>GSHMNILVTGGAGFIGSHVVDKLIENGYGVIVVDNLSSGKVENLNRNALFYEQSIEDEEMMERIFSLHRPEYVFHLAAQASVAISVREPARDAKTNIIGSLVLLEKSIKYGVKKFIFSSTGGAIYGENVKVFPTPETEIPHPISPYGIAKYSTEMYLEFFAREYGLKYTVLRYANVYGPRQDPYGEAGVVAIFTERMLRGEEVHIFGDGEYVRDYVYVDDV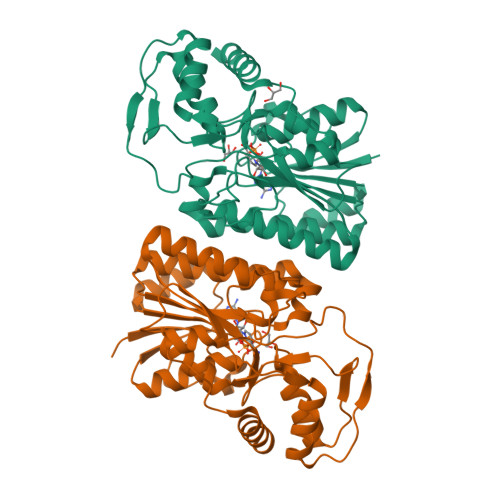VRANLLAMEKGDNEVFNIGTGRGTTVNQLFKLLKEITGYDKEPVYKPPRKGDVRKSILDYTKAKEKLGWEPKVSLEEGLKLTVEYFRKTLE[2x]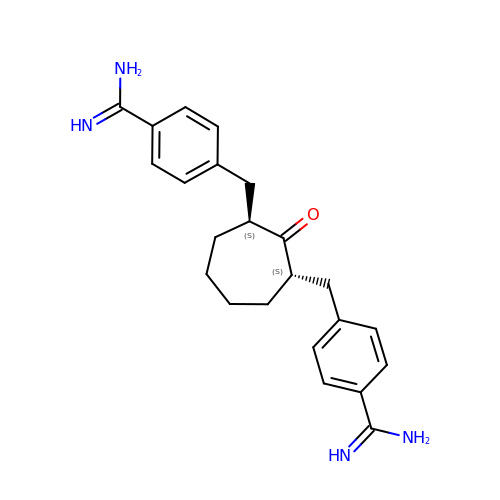2,7-BIS-(4-AMIDINOBENZYLIDENE)-CYCLOHEPTAN-1-ONE | C23 H28 N4 O | BXYGSMRTHHSAHZ-PMACEKPBSA-N> SGTTNTVAAYNLTWKSTNFKTILEWEPKPVNQVYTVQISTKSGDWKSKCFYTTDTECDLTDEIVKDVKQTYLARVFSYPAGNVESTGSAGEPLYENSPEFTPYLETNLGQPTIQSFEQVGTKVNVTVEDERTLVRRNNTFLSLRDVFGKDLIYTLYYWKSSSSGKKTAKTN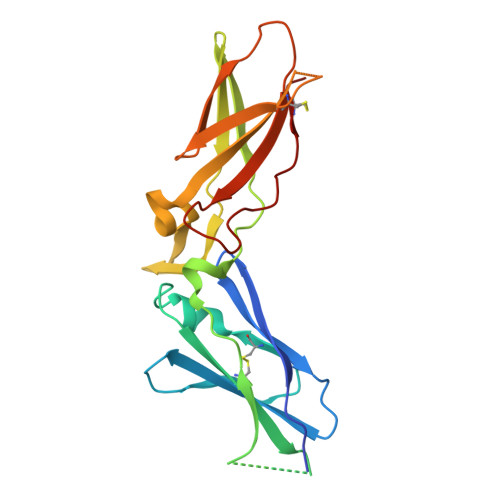TNEFLIDVDKGENYCFSVQAVIPSRTVNRKSTDSPVECMG>GALPDLKIEKLEEGVFVHTSFEEVNGWGVVTKHGLVVLVNTDAYLIDTPFTATDTEKLVNWFVERGYEIKGTISSHFHSDSTGGIEWLNSQSIPTYASELTNELLKKSGKVQAKYSFSEVSYWLVKNKIEVFYPGPGHTQDNLVVWLPESKILFGGCFIKPHGLGNLGDANLEAWPKSAKILMS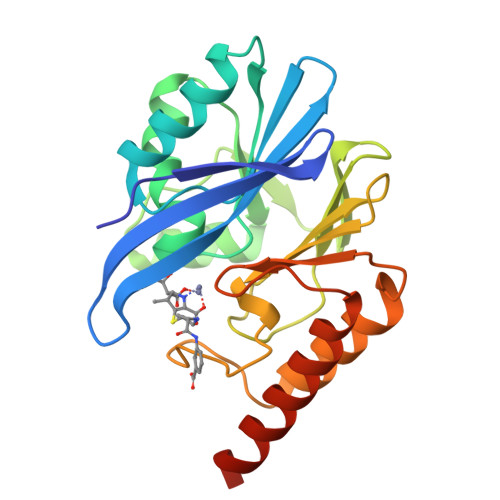KYGKAKLVVSSHSEKGDASLMKRTWEQALKGLKESKKTSSPSN[2x]(3R)-1-(naphthalen-2-ylsulfonyl)piperidine-3-carboxylic acid | C16 H17 N O4 S | 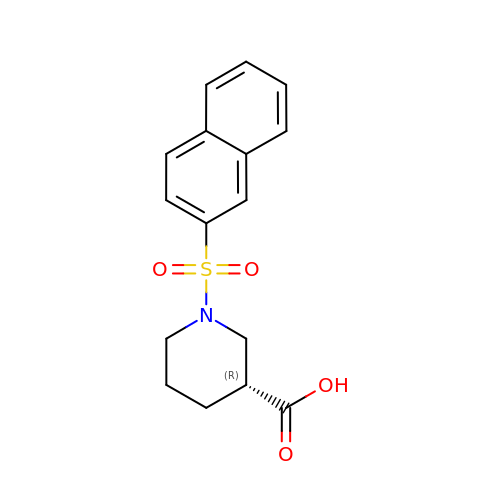KTQWWYGLWQVHDM-CQSZACIVSA-N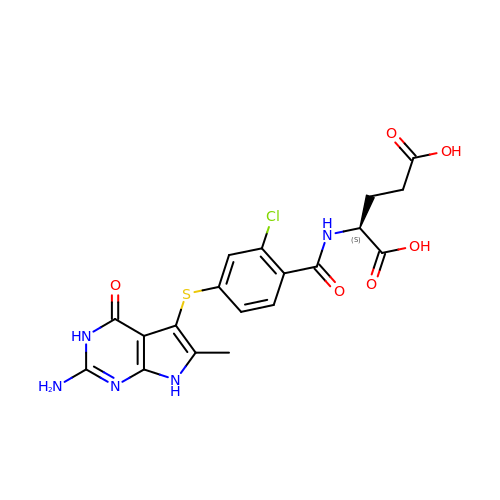N-{4-[(2-amino-6-methyl-4-oxo-4,7-dihydro-3H-pyrrolo[2,3-d]pyrimidin-5-yl)sulfanyl]-2-chlorobenzoyl}-L-glutamic acid | C19 H18 Cl N5 O6 S | DTVBRZFMWHDIOO-NSHDSACASA-N>MEEKIKELEEKVEELVKEALEKKDPAVLKKALVCVYEMKKLGMPNEKLIELLKKLVEVLKKLALERVDPAVLDLALVCVYEMKELGMPNEELIKLLKELVEVLRILALINVDPAVLDKALVCVYLMKELGMPNEELIKLLEELVEVLRILALIRVDKRVLDKAEVCIEEMEELGM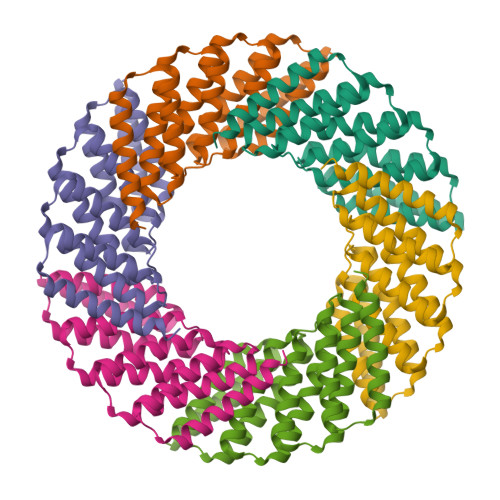PEEKIKELREELKFVREILDKIGSWLEHHHHHH[6x]> KPKLLNKFDKTIKAELDAAEKLRKRGKIEEAVNAFKELVRKYPQSPRARYGKAQCEDDLAEKRRSNEVLRGAIETYQEVASLPDVPADLLKLSLKRRSDRQQFL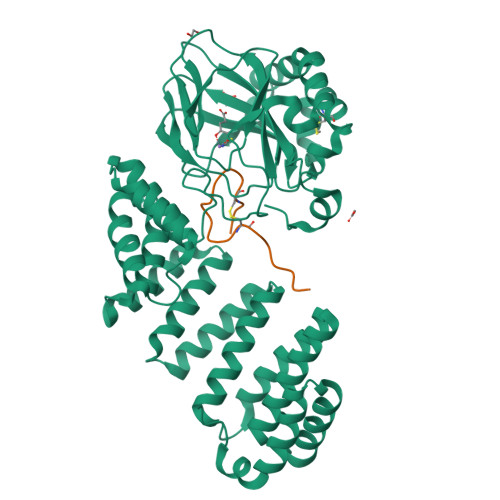GHMRGSLLTLQRLVQLFPNDTSLKNDLGVGYLLIGDNDNAKKVYEEVLSVTPNDGFAKVHYGFILKAQNKIAESIPYLKEGIESGDPGTDDGRFYFHLGDAMQRVGNKEAYKWYELGHKRGHFASVWQRSLYNVNGLKAQPWWTPKETGYTELVKSLERNWKLIRDEGLAVMDKAKGLFLPEDENLREKGDWSQFTLWQQGRRNENACKGAPKTCTLLEKFPETTGCRRGQIKYSIMHPGTHVWPHTGPTNCRLRMHLGLVIPKEGCKIRCANETKTWEEGKVLIFDDSFEHEVWQDASSFRLIFIVDVWHPELTPQQRRSLPAI;> DGDQSETSPSQNQGKCKNGLGEYTCTSLEGFEGKNSELF>GMSSNLHGIAIGIERSQDDFYLAFKAVGKLTHEDYEQMTPLLESALAGIKTPEIVALIDITELDGLSLHAAWDDLKLGLKHGKEFKRVAIIG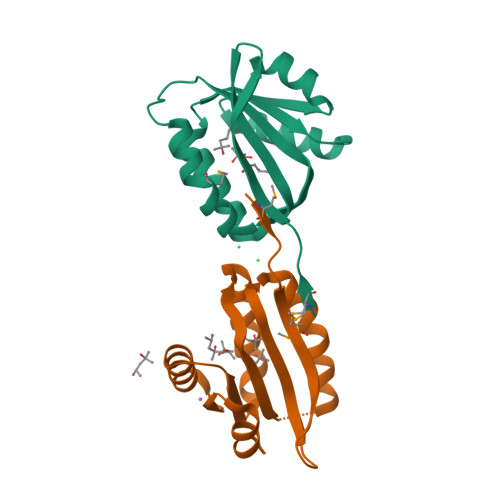QGELQEWATRVANWFTPGEFKFFEDKRDALDWLC[2x]> SSQPNATLYKMSSINADFAFNLYRRFTVETPDKNIFFSPVSISAALVMLSFGACCSTQTEIVETLGFNLTDTPMVEIQHGFQHLICSLNFPKKELE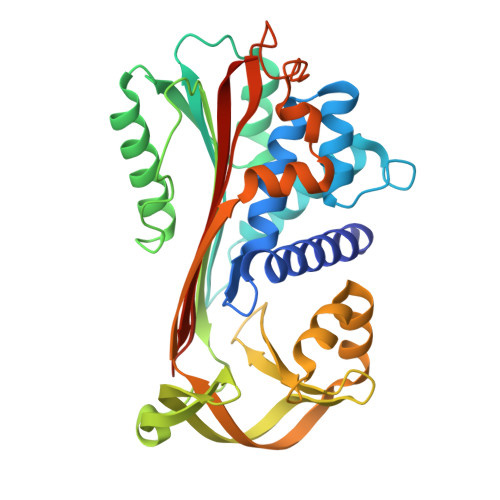LQIGNALFIGKHLKPLAKFLNDVKTLYETEVFSTDFSNISAAKQEINSHVEMQTKGKVVGLIQDLKPNTIMVLVNYIHFKAQWANPFDPSKTEDSSSFLIDKTTTVQVPMMHQMDQYYHLVDMELNCTVLQMDYSKNALALFVLPKEGQMESVEAAMSSKTLKKWNRLLQKGWVDLFVPKFSISATYDLGATLLKMGIQHAYSENADFSGLTEDNGLKLSNAAHKAVLHIGEKGTEAAGAMFLEAIPRSIPNTF>MGKLFGTFGVRGIANEEITPEFALKIGMAFGTLLKREGRERPLVVVGRDTRVSGEMLKDALISGLLSTGCDVIDVGIAPTPAIQWATNHFNADGGAVITASHNPPEYNGIKLLEPNGMGLKKEREAIVEELFFSEDFHRAKWNEIGELRKEDIIKPYIEAIKNRVDVEAIKKRRPFVVVDTSNGAGSLTLPYLLRELGCKVVSVNAHPDGHFPARNPEPNEENLKGFMEIVKALGADFGVAQDGDADRAVFIDENGRFIQGDKTFALVADAVLRENGGGLLVTTIATSNLLDDIAKRNGAKVMRTKVGDLIVARALLENNGTIGGEENGGVIFPDFVLGRDG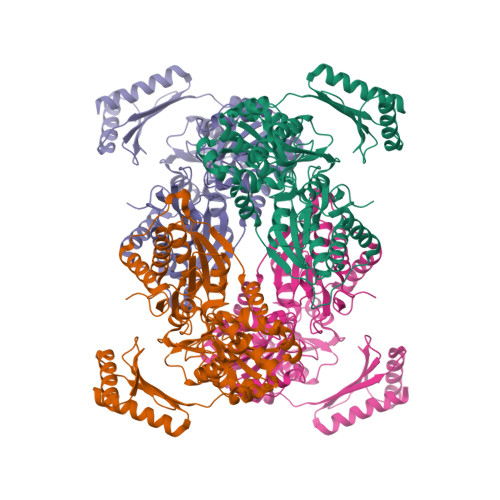AMTTAKIVEIFAKSGKKFSELIDELPKYYQFKTKRHVEGDRKAIVAKVAELAEKKGYKIDTTDGTKIIFDDGWVLVRASGTEPIIRIFSEAKSEEKAREYLELGIKLLEEALKG[4x]>[2x]PMSRAYDLVVLGAGSGGLEAGWNAAVTHKKKVAVVDVQATHGPPLFAALGGTCVNVGCVPKKLMVTGAQYMDLIRESGGFGWEMDRESLCPNWKTLIAAKNKVVNSINESYKSMFADTEGLSFHMGFGALQDAHTVVVRKSEDPHSDVLETLDTEYILIATGSWPTRLGVPGDEFCITSNEAFYLEDAPKRMLCVGGGYIAVEFAGIFNGYKPCGGYVDLCY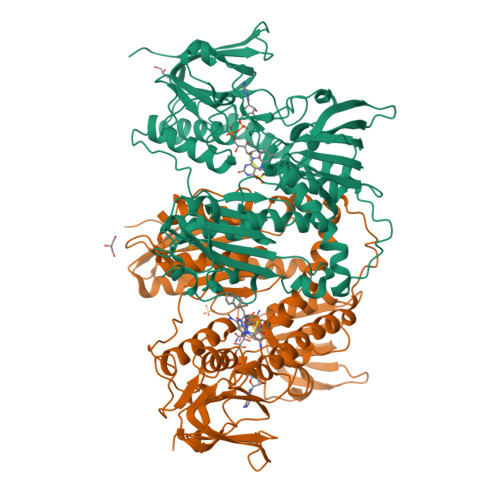RGDLILRGFDTEVRKSLTKQLGANGIRVRTNLNPTKITKNEDGSNHVHFNDGTEEDYDQVMLAIGRVPRSQALQLDKAGVRTGKNGAVQVDAYSKTSVDNIYAIGDVTNRVMLTPVAINEGAAFVETVFGGKPRATDHTKVACAVFSIPPIGTCGMTEEEAAKNYETVAVYASSFTPLMHNISGSKHKEFMIRIITNESNGEVLGVHMLGDSAPEIIQSVGICMKMGAKISDFHSTIGVHPTSAEELCSMRTPAYFYESGKRVEKLSSNL The human nucleoporin Nup98 forms fusion proteins in certain types of malignant leukaemia, is a critical component of the permeability barrier of the nuclear pore complex and is mislocalized in cytosolic deposits in Alzheimer’s disease. Key to these Nup98 activities is its large FG-repeat domain with a high number of FG motifs. The most aggregation-prone segment comprises residues 85–124 (named Nup98FG85). All four fibril types display a parallel in-register β-structure comprising short and kinked β-strands.

To gain insight into the molecular organization of cohesive FG-repeat interactions, Nup98FG85 was allowed to aggregate in pure water. EM revealed the formation of well-defined and mostly separated amyloid fibrils. Using cryo-EM, we determined the structures of four different fibril polymorphs (pm1–pm4). Polymorphs pm2 and pm3, which are almost equally populated, were solved at a resolution of 3.3 and 2.8 Å, respectively, and are formed by two protofilaments. The most common motif shared by the four polymorphs is a 13-residue β-turn/β-arch structure. A leucine-phenylalanine pair (L91-F92) is located at the tip of the β-turn, with both side chains pointing away from the turn. The other LF motifs in the four fibril structures show a very similar structure. In all four Nup98FG85 fibril structures, side chains stacked along the fibril axes build glutamine and asparagine ladders (top). Most of the stabilizing interactions arise where there are clusters of two to four phenylalanine rings and one or more leucine side chains. We obtained values of approximately −20 kcal mol–1 per chain for the four Nup98FG85 fibril structures.

>TGTANTLFGTASTGTSLFSSQNNAFAQNKPTGFGNFGTST[22x]> MCAVLRQPKCVKLRALHSACKFGVAARSCQELLRKGCVRFQLPMPGSRLCLYEDGTEVTDDCFPGLPNDAELLLLTAGETWHGYVSDITRFLSVFNEPHAGVIQAARQQLSDEQAPLRQKLLADLLHHVSQNITAETREQDPSWFEGLESRFRNKSGYL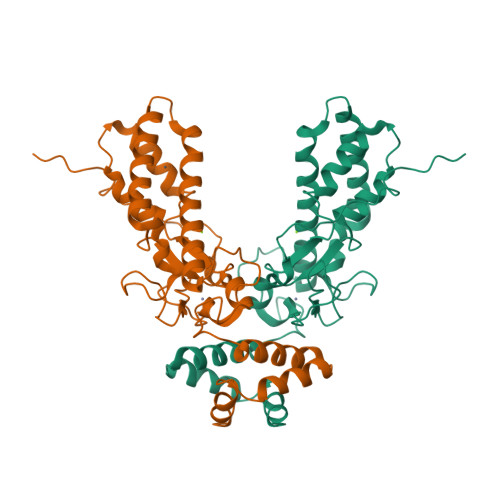RYSCESRIRGYLREVSAYTSMVDEAAQEEYLRVLGSMCQKLKSVQYNGSYFDRGAEASSRLCTPEGWFSCQGPFDLESCLSKHSINPYGNRESRILFSTWNLDHIIEKKRTVVPTLAEAIQDGREVNWEYFYSLLFTAENLKLVHIACHKKTTHKLECDRSRIYRPQTGS> MARKTKEESQKTRDGILDAAERVFLEKGVGTTAMADLADAAGVSRGAVYGHYKNKIEVCLAMCDRAFGQIEVPDENARVPALDILLRAGMGFLRQCCEPGSVQRVLEILYLKCERSDENEPL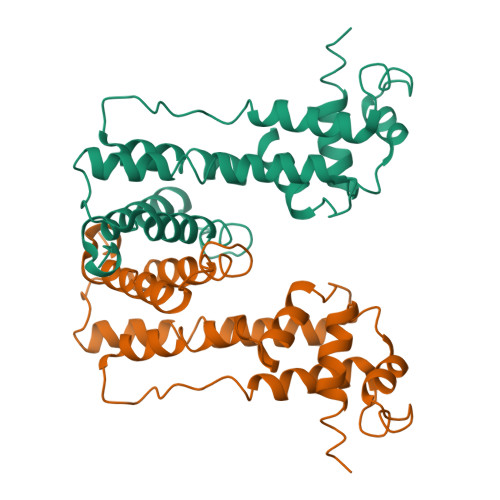LRRRELLEKQGQRFGLRQIRRAVERGELPARLDVELASIYLQSLWDGICGTLAWTERLRDDPWNRAERMFRAGLDSLRSSPYLLLADA> MQNEKLDHESVTQAMQPKDTPELRALYKSFEEESIIPLWTQLGDLMPIHPKSKAVPHVWKWSTLLRLARKSGELVPVGRGGERRHLGLANPGLGGNAYISPTMWAGIQYLGPRETAPEHRHSQNAFRFVVEGEGVWTVVNGDPVRMSRGDLLLTPGWCFHGHMNDTDQPMAWIDGLDIPFSQQMDVGFFEFGSDRVTDYATPNFSRGERLWCHPGLRPLSGLQNTVASPIGAYRWEFTDRALTEQLLLEDEGQPATVAPGHAAIRYVNPTTGGDVMPTLRCEFHRLRAGTETAT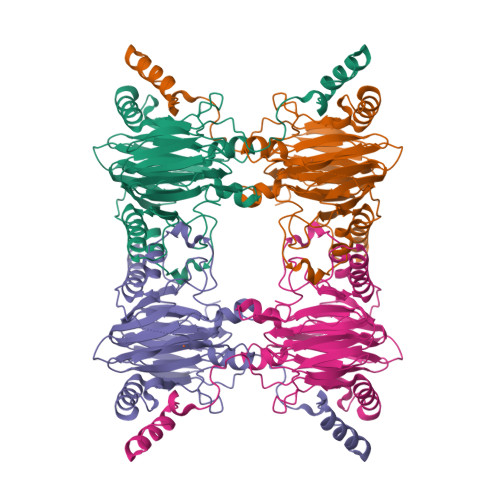RNEVGSTVFQVFEGAGAVVMNGETTKLEKGDMFVVPSWVPWSLQAETQFDLFRFSDAPIMEALSFMRTKIEGQ>[3x]ADPASEEVMACLRQERSRVENPSQTIVNVVAEN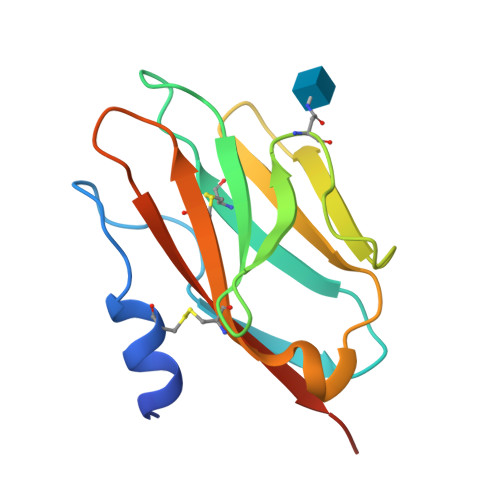PAYLHCSVPPDAEHEIAWTRVSDGALLTAGNRTFTRDPRWQVSKKSANIWVLNLRRAEQQDSGCYLCEINDKHNTVYAVYLKVLEPHHHHHH> MLSFLGKSVALLAALQATLSSPKPGHRRASVEKRANGYANSVYFTNWGIYDRNFQPADLVASDVTHVIYSFMNLQADGTVISGDT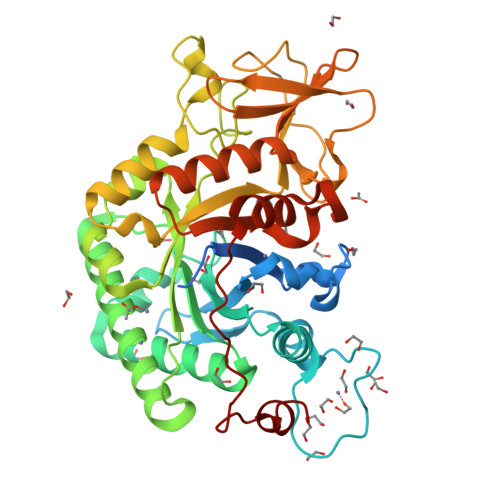YADYEKHYADDSWNDVGTNAYGCVKQLFKVKKANRGLKVLLSIGGWTWSTNFPSAASTDANRKNFAKTAITFMKDWGFDGIDIDWEYPADATQASNMILLLKEVRSQLDAYAAQYAPGYHFLLTIAAPAGKDNYSKLRLADLGQVLDYINLMAYDYAGSFSPLTGHDANLFNNPSNPNATPFNTDSAVKDYINGGVPANKIVLGMPIYGRSFQNTAGIGQTYNGVGSGSWEAGIWDYKALPKAGATVQYDSVAKGYYSYNSATKELISFDTPDMINTKVAYLKSLGLGGSMFWEASADKKGADSLIGTSHRALGGLDTTQNLLSYPNSKYDNIKNGLN>GPLGSSTMGQVGRQLAIIGDDINRRYDSEFQTMLQHLQPTAENA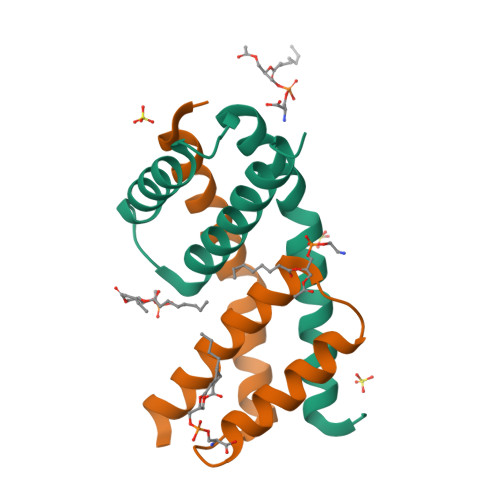YEYFTKIATSLFESGINWGRVVALLGFGYRLALHVYQHGLT[12x]>[3x]ANINDKRVMKEAN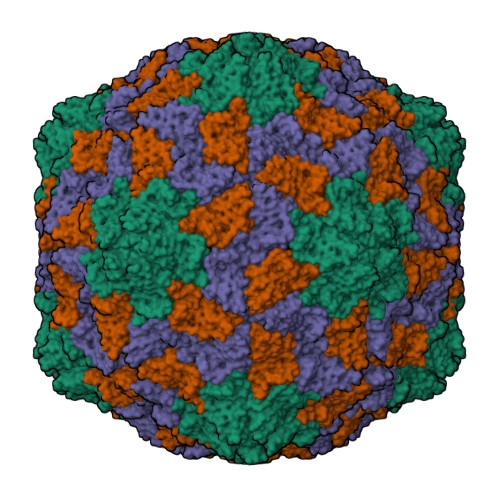GIFVEQRWNGKRWVTEASWRAGQAPNKERAATVTKSIARKVRGGVSRAGGFVTAPVIGAMVTRPTVPRFGMRGNSTVVSNSELILNLTPIALAYTVQSLPLIATQPAWLGTIADNYSKWRWVSLRIIYSPKCPTTTSGTVAMCLSYDRNDVAPGSRVQLSQTYKAINFPPYAGYDGAAILNTDVTPTSAIYVDVDVTRFDKAWYSTIGTAAFAALTAFDQNQFCPCTVHIGSDGGPAVAVPPGDIFFKYVIELIEPINPTMNV>[2x]ASAWPEEKNYHQPAILNSSALRQIAEGTSISEMWQN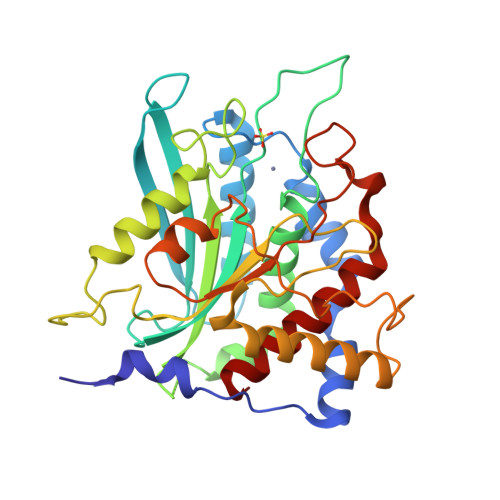DLQPLLIERYPGSPGSYAARQHIMQRIQRLQADWVLEIDTFLSQTPYGYRSFSNIISTLNPTAKRHLVLACHYDSKYFSHWNNRVFVGATDSAVPCAMMLELARALDKKLLSLKTVSDSKPDLSLQLIFFDGEEAFLHWSPQDSLYGSRHLAAKMASTPHPPGARGTSQLHGMDLLVLLDLIGAPNPTFPNFFPNSARWFERLQAIEHELHELGLLKDHSLEGRYFQNYSYGGVIQEDHIPFLRRGVPVLHLIPSPFPEVWHTMDDNEENLDESTIDNLNKILQVFVLEYLHL4-{[(2R,3R)-1,3-dihydroxybutan-2-yl]amino}-6-phenylpyrrolo[1,2-b]pyridazine-3-carboxamide 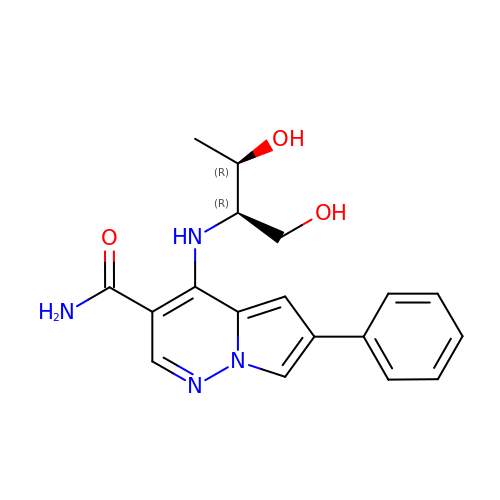| C18 H20 N4 O3 | PRWQQLFMBINSAW-IAQYHMDHSA-N>[2x]MTTRTTDNPWLDARVLNMAHAGGENEAPANTLYAFKRAVKLGANMLELDVQSTKDDQLVVIHNATVDQTTDGTGKVRDLTFEQVHELDAAYNFIPGRHAVPGEPPESYPLRGVRTGEKKPPPGYQPSDFAIPKLADVLEAFPRTPINIEIKGTSDADIPSFLHNAKLLARLLKKTGRTDFIVTSFNDLAVAKFHLLAPDIPIAPGMAGLAAYF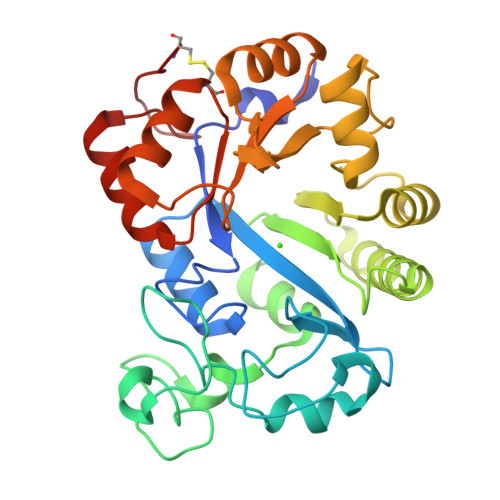LLGVKPMHGTVALQIPVRYQGLEIATPEFIRRAHADGYAVHVWFSGTAPDDEATYNRIIDSCADGLMPAYPALLERILDERGIERPGRPGVDPCG> RTDCYGNVNRIDTTGASCKTAKPEGLSYCGVPASKTIAERDLKAMDRYKTIIKKVGEKLCVEPAVIAGIISRESHAGKVLKNGWGDRGNGFGLMQVDKRSHKPQGTWNGEVHITQGTTILTDFI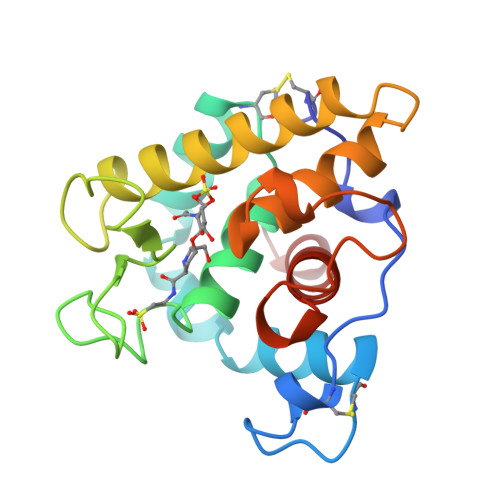KRIQKKFPSWTKDQQLKGGISAYNAGAGNVRSYARMDIGTTHDDYANDVVARAQYYKQHGY> MSKQQYRLGIDAGGTFTDFILADHQGNVQLFKAPSTPHDGTLAIRNGLAQIADALGRTPAEIIADCDLCINGTTVALNALIEKTGVKVGLLCTDGHEDSLEIRLGHKEDGHRYDATYPPAHMLVPRHLRRPIGGRIISDGSEFSPLDEAAIHAAIDYFREQQVQAVAISFVWSVRNPSHEQRAMAMVRAALPDVFVCSGHEVFPQIREYTRTSTTVVNAYLSPVMGRYIERIDALFEELGAQQPTRYFQSNGGLAPGVVMRERAVNAINSGPASAPQAGLCVAQPFGIDNVITVDMGGTSFDITLSKGGRTNFSKDSDFLRYRIGVPMIQVETLGAGGGSIAHLDDFGMLQVGPRSAGANPGPVCYGKGGVEPTVTDANLALGYLADGALLGGSIRLNRQAAIDAIRSKIAEPLGISVERAAVGIITLVNLSMVSGIRRVSIERGYDPRDFALIGAGGAAGMHVMRLAEEIGSKVVLIPKVASGLCAFGQILSDIRYDQLTTLPMRLDDEFVDLEQLNQALQQLRERGMTNLRDDGFGGDNRIECQYSLEIRYLGQIHECSVELSCDRLDR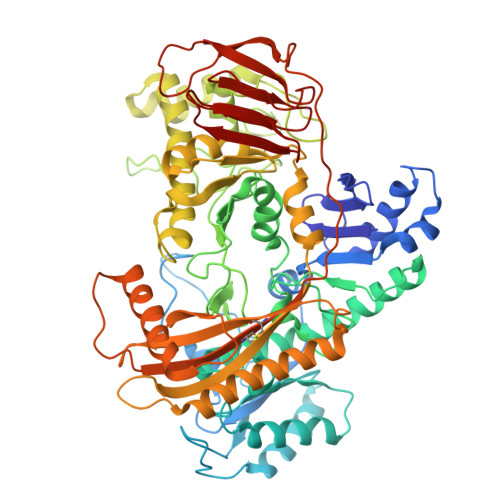SSLAALRESFHQRHKALFSYSEPNSPVELVNLECSVIARLQRPPMPELATPLKATAAIPAGHRPMLFNAQDDWQDTPVYNGDRIEVGQIIQGPCVIEEATTNILVPPGWRVSLDPSATYELTPGH Fungal carbonic anhydrases (CAs) are metalloenzymes that catalyze the reversible hydration of carbon dioxide and play an essential role in fungal adaptation to environments with fluctuating CO2 concentrations. The opportunistic pathogen Candida parapsilosis expresses a single β-class CA, CpNce103p, which is structurally distinct from human α-class CAs and therefore may represent a promising antifungal target. Mass photometry and X-ray crystallography revealed that CpNce103p forms a stable homotetramer, similar to its homolog CaNce103p from C. albicans. In summary, CpNce103p shares fundamental structural features with other fungal β-CAs – a tetrameric assembly, the Cys–His–Cys zinc site, and a funnel-shaped active-site channel – while differing mainly in peripheral regions.

However, only the Δ42 construct, which fully excludes the predicted disordered region and C-terminal tail, yielded well-diffracting crystals. The crystal structure of CpNce103p in complex with acetazolamide (AZM) reveals a homotetramer organized as a dimer of dimers. Consistent with this, the active site of each monomer is positioned near the dimer interface, with the neighboring subunit contributing certain active-site residues. Each monomer in the tetramer is bound to one AZM molecule (one inhibitor per active site), yielding a fully occupied tetramer with four bound inhibitors. In the AZM-bound CpNce103p structure, Zn2+ is tetrahedrally coordinated by Cys81A, His136A, Cys139A, and the sulfonamide nitrogen of AZM. The sulfonamide group replaces the catalytic water as the fourth Zn2+ ligand. Key contributions include His136A and Asp83A from chain A, and Gln72B and Phe121B from chain B. AZM forms several hydrogen bonds. Its sulfonamide NH− group donates an H-bond to Asp83A, while one sulfonyl oxygen accepts an H-bond from Gln72B. The other sulfonyl oxygen interacts with the backbone NH groups of Ala105A and Gly141A. Hydrophobic and aromatic interactions further reinforce binding. The thiadiazole ring of AZM engages in a π–π stacking interaction with Phe121B from the adjacent subunit (∼3.8 Å), while surrounding nonpolar residues form additional van der Waals contacts. The C-terminus of CpNce103p is disordered in our structure: no density corresponding to an expected helix (often labeled “α12” in homologous structures) was observed.

>[4x]VTSHSNFPFTLSPDSTITDYLNNNKFYVDSIKHNHGDQIFELNGKGQSPHTLWIGCSDSRAGEQCLATLPGEIFVHRNIANIVNSNDFSSQGVIQFAIDVLKVKKIIVCGHTDCGGIWASLSSKKIGGVLDLWLNPVRHIRAQNLKLLEQYNHEPKLKARKLAELNVIASVIALKRHPSASTALKQGKIEVWGMIYDVASGYLSELEIPQDEFHELFHVLDEEDASAHNAH> TEETITIDSISNGILNNLLTTL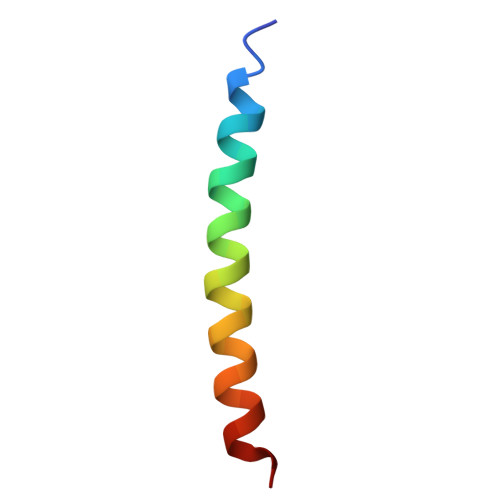IQDIVARETT> SDKELKFLVVDDFSTMRRIVRNLLKELGFNNVEEAEDGVDALNKLQAGGYGFVISAWNMPNMDGLELLKTIRADGAMSALPVL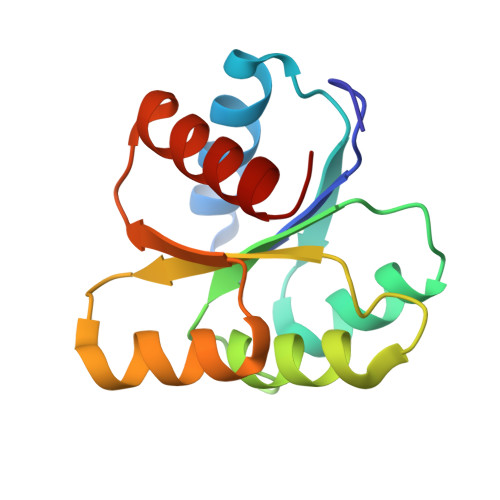MVTAEAKKENIIAAAQAGASGYVVKPFTAATLEEKLNKIFEKLGM> MAQSVTADPSPPITDTNKLNKYSSRITEPKSQGGSQAILHGVGLSDDDLLKPQIGISSVWYEGNTCNMHLLKLSEAVKEGVENAGMVGFRFNTIGVSDAISMGTRGMCFSLQSRDLIADSIETVMSAQWYDGNISIPGCDKNMPGTIMAMGRLNRPGIMVYGGTIKPGHFQDKTYDIWSAFQSYGEFVSGSISDEQRKTVLHHSCPGAGACGGMYTANTMASAIEAMGMSLPYSSSIPAEDPLKLDECRLAGKYLLELLKMDLKPRDIITPKSLRNAMVSVMALGGSTNAVLHLIAIARSVGLELTLDDFQKVSDAVPFLADLKPSGKYVMEDIHKIGGTPAVLRYLLELGLMDGDCMTVTGQTLAQNLENVPSLTEGQEIIRPLSNPIKETGHIQILRGDLAPDGSVAKITGKEGLYFSGPALVFEGEESMLAAISADPMSFKGTVVVIRGEGPKGGPGMPEMLTPTSAIMGAGLGKECALLTDGRFSGGSHGFVVGHICPEAQEGGPIGLIKNGDIITIDIGAARIDTQVSPEEMNDRRKKWTAPAYKVNRGVLYKYIKNVQSASDGCVTDE

Dihydroxy acid dehydratase (DHAD) is the third enzyme in the plant branched-chain amino acid biosynthetic pathway and the target for commercial herbicide development. We have previously reported the discovery of fungal natural product aspterric acid (AA) as a submicromolar inhibitor of DHAD through self-resistance gene directed genome mining. Here, we reveal the mechanism of AA inhibition on DHAD and the self-resistance mechanism of AstD, which is encoded by the self-resistance gene astD. Our structural and kinetic analysis of the mutant AthDHADs has validated the hypothesis that larger hydrophobic amino acids surrounding the active-site entrance enhance resistance to AA.

Furthermore, we also generated mutants of V178, which was shown to interact with the isopropylcyclopentane portion of AA in the AthDHAD–AA complex structure. The AA resistance of all V178 mutants were increased, where the IC50 values were 0.97, 0.43, 6.00, and 2.34 μM for V178L, V178I, V178F, and V178W mutants, respectively. The observed increases in IC50 suggest that the larger hydrophobic side chains of these mutants effectively narrowed the entrance to the active site, thereby impeding the entry of AA into the catalytic region. To probe the acquired resistance mechanism of AthDHAD mutants, we determined the crystal of AthDHAD–I177F (2.45 Å), AthDHAD–V178W (1.77 Å), AthDHAD–V496W (1.59 Å), and AthDHAD–V497F (1.87 Å). In the crystal structures of I177F, V178W, V496W, and V497F, the occupancy of [2Fe–2S] cluster is 0.64, 0.72, 0.63, and 0.77, respectively. The overall structures of the AthDHAD mutants I177F, V178W, V496W, and V497F displayed high similarity with the wild-type AthDHAD, with the RMSD of 0.123 Å (888 core Cα atoms), 0.275 Å (994 core Cα atoms), 0.142 Å (1,034 core Cα atoms), and 0.283 Å (994 core Cα atoms), respectively. As a result, this mutant also affects the accession of AA to the active site. Both V178 and I177 are close to the active site. Alignment of the AthDHAD–AA complex structure to V178W reveals that the side chain of W178 has 2 conformations and not only makes the channel entrance narrower but also occupies the position of isopropylcyclopentane of AA.>[6x]SIVTKSIVNADAEARYLSPGELDRIKSFVSGGAQRLRIAQVLTDNRERIVKQAGDQLFQKRPDVVSPGGNAYGQE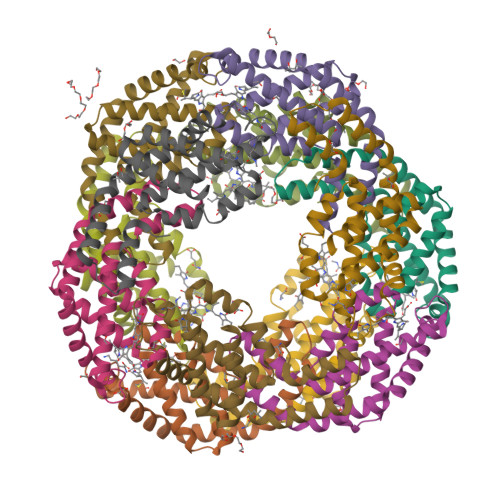MTATCLRDLDYYLRLVTYGIVAGDVTPIEEIGIVGVREMYKSLGTPIDAVAGGVAAMKSVAAGLLSAEDAGEAGAYFDYVVGAMQ;>MQDAITSVINSSDVQGKYLDNAALEKLKGYFATGELRVRAATTISANAAAIVKEAVAKSLLYSDITRPGGNMYTTRRYAACIRDLDYYLRYATYAMLAGDPSILDERVLNGLKETYNSLGVPVGATVQAIQAIKEVTASLVGPDAGKEMGVYFDYICSGLS[6x]(3-CHLORO-4-PROPOXY-PHENYL)-ACETIC ACID | C11 H13 Cl O3 | 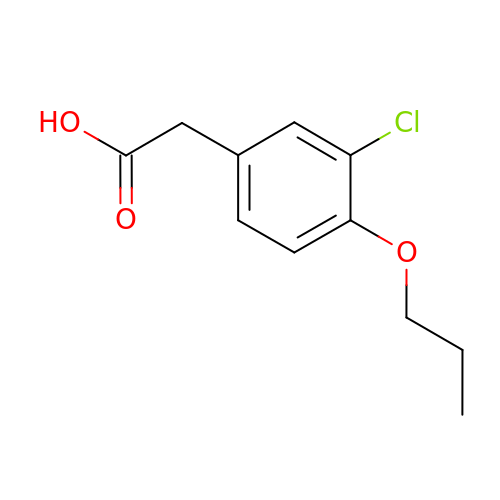QEJHPAGTOOIBFT-UHFFFAOYSA-N>[18x]MVRKVFNDGDILYAEDVNIIGQPFVDGQDLLGHGLKVDDNSLSDEPQNIKTRFYAWYNRFRVTVQSGLTLSVTQGSISVSGNIISFPPQTINAIDNANSFVWIGKTDADPAIALRVSQTLPNVCIPLARVIAASGSVTSVTDLRDVSVDILPPSIPDAVPVGSTIISLIPPTAPIPAGYLELL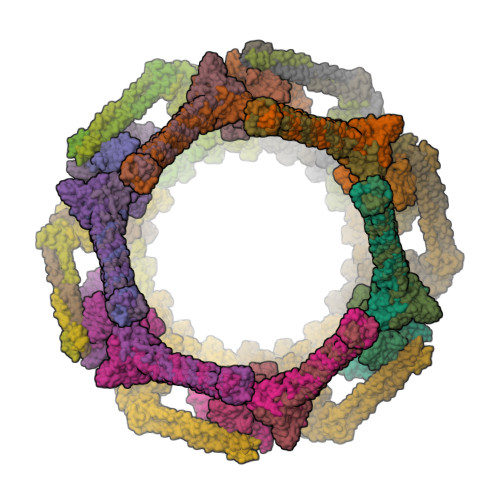NSSQNVSRTTYSALFVLWGTYYGNGDGSTTFGVPGTGGRFLRLGGSGLSVGDIGGSNQITIPTNALPSHQHGIPANTHTHSVNDGGHGHTINQTPHSHSISDPGHAHGVPFGAAVDNGNNAFDTGGSPYNNGIGTTQNQTGISVNTANANLSINTSSTGISIQSASTGLTVTSNAGNGQAFQHDQPYLVFRVFVKV;>MTNIVGRIGFLTTGKLGIKLRGVLIDESTTPNTTYLPGIESFFNITANVLTSVSYPETETQNVTATFSIYSVDGSSNPVFPALLSFDAIVPNVASVEFDVLAPTGVVNNQLDTSALRIAKIIANDPALAQKVAGAPYPRGAYSATETYLYGEMVSYFGKNYISKSLSPIINILPTVTDSWYELVITLPESVSVIATGSDTAYGTGWNGSLLVPTQNAVYDKIVTVDAAIATANTNITNLGTAKADLSYVNTQLSADQVVLDALSSGKADLSYVNTQLNSKANLNGAVLVNATTATPPISDNDTSLATTQHVRSFNHSRLAFNAFRGGQQGVPSLSYVTTTAQFNSSSVRSGWGDNFSSNRWLVGEGGTYLITVTTRFATVGGTPPTYFDALLFVGLSGSGVENFLTRSQSVYPSFGYTLSWVGILTFNTGQNVFLNYQVNAVGGGSYSVVLEDVRFSGIQLG[18x]> EQAPQYVDETISLSAKTLFGFDKDSLRAEAQDNLKVLAQRLSRTNIQSVRVEGHTDFMGSDKYNQALSE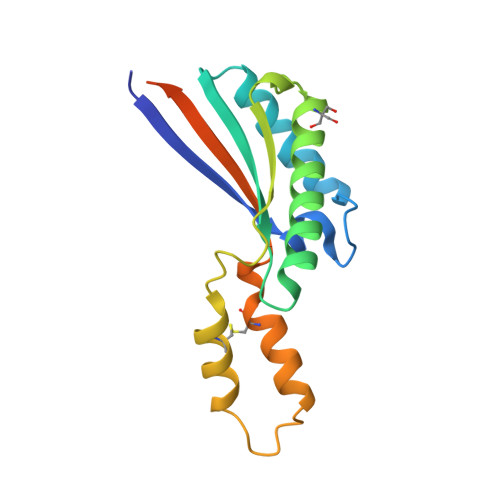RRAYVVANNLVSNGVPVSRISAVGLGESQAQMTQVCEAEVAKLGAKVSKAKKREALIACIEPDRRVDVKIRSIVTRQVVPAHNHHQHLEHHHHHH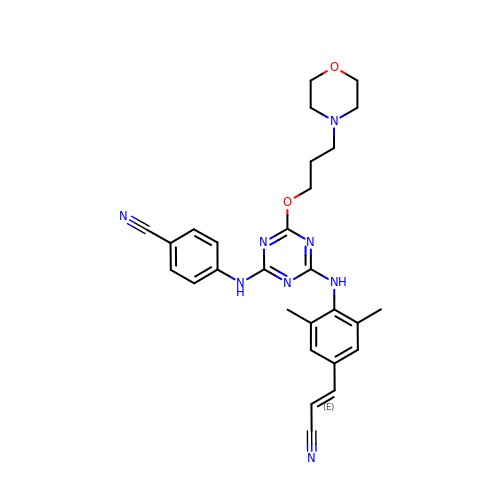4-[(4-{4-[(E)-2-cyanoethenyl]-2,6-dimethylanilino}-6-[3-(morpholin-4-yl)propoxy]-1,3,5-triazin-2-yl)amino]benzonitrile | C28 H30 N8 O2 | IRRZMAXYIYCORM-HWKANZROSA-N> MYKILEIADVVKVPPEEFGKDLKETVKKILMEKYEGRLDKDVGFVLSIVDVKDIGEGKVVHGDGSAYHPVVFETLVYIPEMYELIEGEVVDVVEFGSFVRLGPLDGLIHVSQIMDDYVSYDP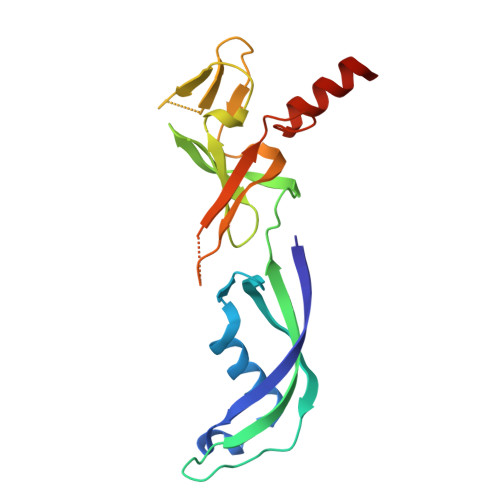KREAIIGKETGKVLEIGDYVRARIVAISLKAERKRGSKIALTMRQPYLGKLEWIEEEKAKKQNQE Carbamate kinase (CK; EC 2.7.2.2, ATP:carbamate phosphotransferase) reversibly converts ADP and carbamoyl phosphate into ATP and ammonium carbamate. The enzyme functions in the L-arginine dihydrolase pathway, operative primarily in some bacteria but also in the enteric protozoan parasite, Giardia lamblia. CK assembles into homodimers, consistent with the oligomeric form detected in solution. Each subunit contains an eight-stranded β-sheet surrounded by three α-helices on one side and four α-helices on the other side of the β-sheet.

An AMP-PNP molecule binds to each of the four subunits within the crystal asymmetric unit. AMP-PNP binds in a pocket flanked by amino acid residues 11–13, 235–250, and 267–278. It exhibits the same interactions whether CK’s auxiliary domain adopts the open conformation or is disordered, as the nucleotide does not interact with the auxiliary domain. Of the two homodimers in the asymmetric unit, the auxiliary domains of only one homodimer adopt the open conformation while those in the second homodimer are structurally disordered. The following interactions are common to both structures. The loop comprising amino acid residues 245–250 undergoes a conformational transition upon AMP-PNP binding such that the side chain of Tyr245 (Tyr238 in efCK) stacks against the adenine ring and its hydroxyl group forms a hydrogen bond with the ribose O2′ hydroxyl group (see Fig. 3C for atom numbering and protein-ligand interactions). Met275 (Met268 in efCK) side chain stacks against the opposite face of the adenine moiety. Present in glCK-AMPPNP but absent in the efCK-ADP structure is a hydrogen bond between the O3′ hydroxyl of the ribose and the carboxyl group of Asp237 (Gly230 is the equivalent residue in efCK). However, no electron density is associated with Mg2+ in the glCK-AMPPNP structure reported here. We therefore propose that although catalytic activity requires the presence of a divalent cation, the metal ion is not required for nucleotide binding in the active site.

>GMSAGKTVVIALGGNAMLQAKEKGDYDTQRKNVEIAASEIYKIHKAGYKVVLTSGNGPQVGAIKLQNQAAAGVSPEMPLHVCGAMSQGFIGYMMSQAMDNVFCANNEPANCVTCVTQTLVDPKDQAFTNPTKPVGRFYTEQEAKDLMAANPGKILREDAGRGWRVVVPSPRPLEIVEYGVIKTLIDNNVLVICTNGGGIPCKRENKVISGVDAVIDKDLATSLLAKTLNSDYLMILTDVLNACINYKKPDERKLEEIKLSEILALEKDGHFAAGSMGPKVRAAIEFTQATGKMSIITSLSTAVDALNGKCGTRIIKD[4x]>MEDINWQLFGPNLYTSMVKIAIPDFFERIRVKGDGNCFFRAFAYLFFDTEEMWDTVKGTALGYARQHWSECHGAKGVYNYRAENEIKSEKALYSSVLRGNATENVTRRGLDLYLEDATKEGYWGGTDEAEMLASALNVTIVIWNVNTDMKVLDVQKFGTDSVPRAFNIVRCGAHFDALKLINQHGTEAATVSTKSGSHHHHHH[2x]

One specific mechanism used by nairoviruses is the production of a deubiquitinating enzyme, termed the vOTU, that disrupts the innate immune response. Interestingly, the nairoviral L segment also encodes a viral homologue of the ovarian tumor protease (OTU) at the N-terminus. Instead, the vOTU’s primary function appears to be the reversal of post-translational modifications by ubiquitin (Ub) and the Ub-like protein interferon stimulated gene product 15 (ISG15). Each vOTU possesses a seven-stranded beta sheet as the core feature, with five major alpha helices framing the rest of the structure.

Viruses in the Hughes orthonairovirus species possess an additional 26–30 amino acids in the middle of the vOTU. To assess how this additional sequence influences the structure of vOTUs in this subset of nairoviruses, a crystal structure of FARV vOTU was solved to 2.22 Å. While possessing the familiar core domain and secondary structure features, the protease possesses extended α3/α4 helices that are connected by several intervening residues. Thirteen residues could not to be built due to a lack of well-defined electron density in the crystal structure, and those that could be modeled possess high B factors, suggesting this region to have a high degree of flexibility. Additionally, the α3/α4 helices of FARV vOTU appear to interact with each other in a manner resembling a coiled-coil motif. This is facilitated by hydrophobic packing between Ile86, Val105, Ala82, and the aliphatic portion of the Arg108 sidechain. Looking at the selectivity pocket of FARV vOTU reveals it to possess more of a hydrophilic character and contains a relatively bulky Gln155 residue in the equivalent site to position 131 in CCHFV. Additionally, FARV vOTU possesses a potential steric hindrance to efficient binding with the presence of Arg170. Removing this region reduced activity towards Ub-AMC by almost 60%, suggesting that this motif could play a significant role in Ub binding.3-[(2-{[(benzyloxy)carbonyl]amino}ethyl)selanyl]-L-alanine 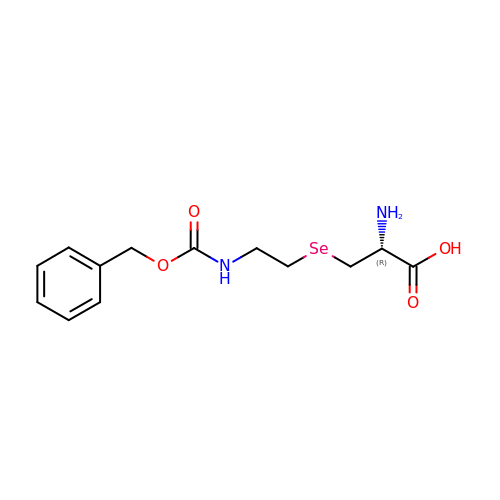| C13 H18 N2 O4 Se | JNNNCAOHWXXURB-NSHDSACASA-N> MLDEALMPKHIALIMDGNRRWAKDKGLDVSEGYKHLFPKLKEICDISSKLGIQVITAFAFSTENWKRAKGEVDFLMQMFEELYDEFSRSGVRVSIIGCKTDLPMTLQKCIALTEETTKGNKGLHLVIALNYGGYYDILQATKSIVNKAMNGLLDVEDINKNLFDQELESKCPNPDLLIRTGGDQRVSNFLLWQLA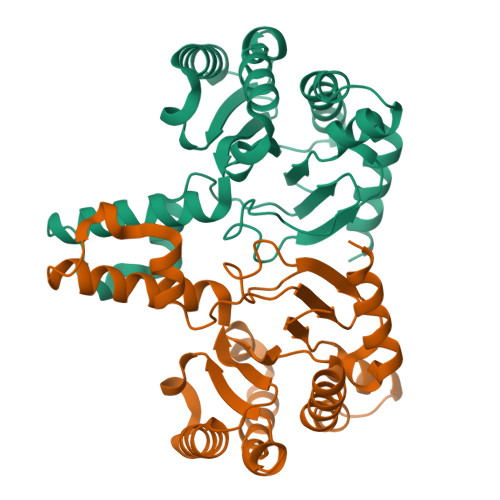YTEFYFTKTLFPDFGEEDLKEAIINFQQRHRRFGGHTY> IVGGYTCAANSIPYQVSLNSGSHFCGGSLINSQWVVSAAHCYKSRIQVRLGEHNIDVLEGNEQFINAAKIITHPNFNGNTLDNDIMLIKLSSPATLNSRVATVSLPRSCAAAGTECLISGWGNTKSSGSSYPSLLQCLKAPVLSDSSCKSSYPGQITGNMICVGFLEGGKDSCQGDSGGPVVCNGQLQGIVSWGY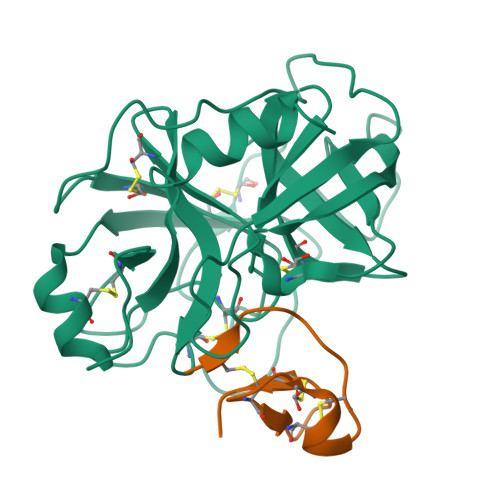GCAQKNKPGVYTKVCNYVNWIQQTIAAN;> GCPRILIRCKQDSDCLAGCVCGPNGFCGSPHHHHHH> LADKVIINTAAVENPSLITQIAQTFGSQAVVVAIDAKRVDGEFMAFTYSGKKNTGILLRDWVVEVEKRGAGEILLASIDRGGTKSGYDTEMIRFVRPLTTLPIIASGGAGKMEHFLEAFLAGADKVSINTAAVENPSLITQIAQTFGSQAVVVAIVAKRVDGEFMVFTYSGKKNTGILLRDWVVEVEKRGAGEILLTSIDRVGTKSGYDTEMIRFVRPLTTLPIIA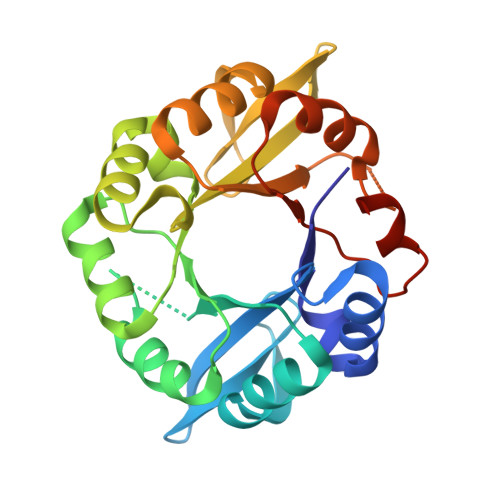SGGAGKMEHFLEAFLAGADA The membrane-anchored SNARE (soluble N-ethylmaleimide-sensitive factor acceptor protein receptor) proteins provide the energy to drive membrane fusion in various cellular contexts, such as intracellular trafficking and exocytosis. Supercomplexes of NSF, α-SNAP, and either a syntaxin tetramer or one of two binary complexes of syntaxin—SNAP-25 reveal atomic details of SNARE processing and show how sequential ATP hydrolysis drives disassembly. NSF comprises three structured domains connected by flexible linkers—the adapter N-domain followed by the D1 and D2 AAA+ domains. Six NSF protomers come together to form the active form of the enzyme, a homo-hexamer.

Even without further processing, this structure was recognizable as a parallel 2:2 syntaxin—SNAP-25 sub-complex formed by two syntaxin H3 SNARE domains and two SNAP-25 SN1 SNARE domains; this binary 2:2 configuration was previously observed in crystal structures of syntaxin-1 H3 and SNAP-25 SN1 domains and was unexpected as we prepared the complex with full-length proteins, implying that two independent SNAP-25 molecules contribute their SN1 SNARE domains to this complex. Presumably, disassembly of the binary 2:1 complex had occurred and was followed by reassembly of the 2:2 binary complex before vitrification. The 2:2 binary complex was fit back into the full reconstructions, enabling modeling of the full 22bin20S. Again, syntaxin is bound within the pore of the D1 ring. Critically, the pore loop approaches the substrate-engaged state found in the non-hydrolyzing classes; together, this suggests a trajectory of protomer A dissociation, nucleotide release and rebinding, and, finally, SNARE substrate rebinding. Furthermore, in classes with ordered syntaxin substrate, the unstructured region of syntaxin N-terminal to the H3 domain is engaged by the D1 pore loops around eight residues further into the primary sequence under hydrolyzing conditions. Of the five 22bin20S classes with the 2:2 binary SNARE complex, all are found with syntaxin in the D1 pore, while two are observed with the N-terminus of the SNAP-25 SN1 domain in the pore. Four ɑ-SNAP molecules bind the 2:2 binary SNARE complex, with two SNAP-25 SN1 SNARE domains and two syntaxin H3 domains. This configuration locates two independent N-terminal portions of the SNAP-25 linker bearing cysteine sidechains often palmitoylated in vivo near the membrane. The 2:2 configuration is only found following NSF-mediated disassembly of the 2:1 configuration.

>[6x]GANMAGRSMQAARCPTDELSLSNCAVVSEKDYQSGQHVIVRTSPNHKYIFTLRTHPSVVPGSVAFSLPQRKWAGLSIGQEIEVALYSFDKAKQCIGTMTIEIDFLQKKNIDSNPYDTDKMAAEFIQQFNNQAFSVGQQLVFSFNDKLFGLLVKDIEAMDPSILKGEPASGKRQKIEVGLVVGNSQVAFEKAENSSLNLIGKAKTKENRQSIINPDWNFEKMGIGGLDKEFSDIFRRAFASRVFPPEIVEQMGCKHVKGILLYGPPGCGKTLLARQIGKMLNAREPKVVNGPEILNKYVGESEANIRKLFADAEEEQRRLGANSGLHIIIFDEIDAICKQRGSMAGSTGVHDTVVNQLLSKIDGVEQLNNILVIGMTNRPDLIDEALLRPGRLEVKMEIGLPDEKGRLQILHIHTARMRGHQLLSADVDIKELAVETKNFSGAELEGLVRAAQSTAMNRHIKASTKVEVDMEKAESLQVTRGDFLASLENDIKPAFGTNQEDYASYIMNGIIKWGDPVTRVLDDGELLVQQTKNSDRTPLVSVLLEGPPHSGKTALAAKIAEESNFPFIKICSPDKMIGFSETAKCQAMKKIFDDAYKSQLSCVVVDDIERLLDYVPIGPRFSNLVLQALLVLLKKAPPQGRKLLIIGTTSRKDVLQEMEMLNAFSTTIHVPNIATGEQLLEALELLGNFKDKERTTIAQQVKGKKVWIGIKKLLMLIEMSLQMDPEYRVRKFLALLREEGASPLDFD;>[2x]MKDRTQELRTAKDSDDDDDVTVTVDRDRFMDEFFEQVEEIRGFIDKIAENVEEVKRKHSAILASPNPDEKTKEELEELMSDIKKTANKVRSKLKSIEQSIEQEEGLNRSSADLRIRKTQHSTLSRKFVEVMSEYNATQSDYRERCKGRIQRQLEITGRTTTSEELEDMLESGNPAIFASGIIMDSSISKQALSEIETRHSEIIKLENSIRELHDMFMDMAMLVESQGEMIDRIEYNVEHAVDYVERAVSDTKKAVKYQSKARRKKIM;>[2x]MGSSHHHHHHSQDPNSMAEDADMRNELEEMQRRADQLADESLESTRRMLQLVEESKDAGIRTLVMLDEQGEQLERIEEGMDQINKDMKEAEKNLTDLGKFAGLAVAPANKLKSSDAYKKAWGNNQDGVVASQPARVVDEREQMAISGGFIRRVTNDARENEMDENLEQVSGIIGNLRHMALDMGNEIDTQNRQIDRIMEKADSNKTRIDEANQRATKMLGSG;>[4x]GMDTSGKQAEAMALLAEAERKVKNSQSFFSGLFGGSSKIEEACEIYARAANMFKMAKNWSAAGNAFCQAAQLHLQLQSKHDAATCFVDAGNAFKKADPQEAINCLMRAIEIYTDMGRFTIAAKHHISIAEIYETELVDVEKAIAHYEQSADYYKGEESNSSANKCLLKVAGYAAQLEQYQKAIDIYEQVGTSAMDSPLLKYSAKDYFFKAALCHFCIDMLNAKLAVQKYEELFPAFSDSRECKLMKKLLEAHEEQNVDSYTESVKEYDSISRLDQWLTTMLLRIKKTIQGDEEDLR>MDQDSLSSSLKTCYKYLNQTSRSFAAVIQALDGEMRNAVCIFYLVLRALDTLEDDMTISVEKKVPLLHNFH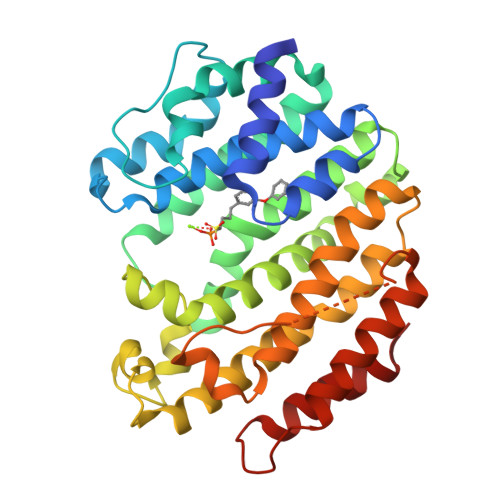SFLYQPDWRFMESKEKDRQVLEDFPTISLEFRNLAEKYQTVIADICRRMGIGMAEFLDKHVTSEQEWDKYCHYVAGLVGIGLSRLFSASEFEDPLVGEDTERANSMGLFLQKTNIIRDYLEDQQGGREFWPQEVWSRYVKKLGDFAKPENIDLAVQCLNELITNALHHIPDVITYLSRLRNQSVFNFCAIPQVMAIATLAACYNNQQVFKGAVKIRKGQAVTLMMDATNMPAVKAIIYQYMEEIYHRIPDSDPSSSKTRQIISTIRTQN[6x]> GSHMTTPSHLSDRYELGEILGFGGMSEVHLARDLRLHRDVAVKVLRADLARDPSFYLRFRREAQNAAALNHPAIVAVYATGEAETPAGPLPYIVMEYVDGVTLRDIVHTEGPMTPKRAIEVIADACQALNFSHQNGIIHRDVKPANIMISATNAVKVMDFGIARAIADSGNSVTQTAAVIGTAQYLSPEQARGDSVDARSDVYSLGCVLY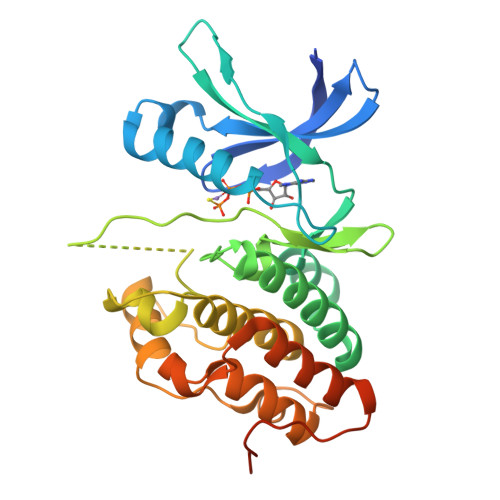EVLTGEPPFTGDSPVSVAYQHVREDPIPPSARHEGLSADLDAVVLKALAKNPENRYQTAAEMRADLVRVHNGEPPEAPKVLTDAERTSLLSSAAGNLSGPR>[2x]MGMLGLDLLKEVPGLLEEIKALPLRLDEERFRFWLQQDYPFVEALYRYQVGLL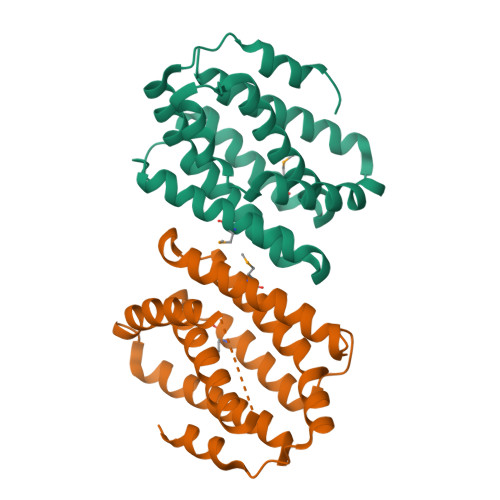LEAPQAHRAPLVQALMATVEELDWLLLQGASPSAPVHPVRAGYIALLEEMGRLPYAYRVVFFYFLNGLFLEAWAHHVPEEGPWAELSQHWFAPEFQAVLYDLEVLARGLWEDLDPEVVRTYLRRILEAEKATWSLLL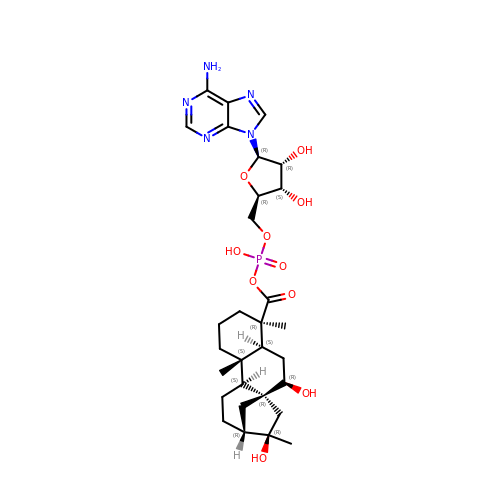5'-O-[(R)-{[(7beta,8alpha,9beta,10alpha,13alpha,16beta)-7,16-dihydroxy-18-oxokauran-18-yl]oxy}(hydroxy)phosphoryl]adenosine | C30 H44 N5 O10 P | LGCUMWKRNQUJBL-BSUNFUJCSA-N>[4x]MKLSGVELRRVQMPLVAPFRTSFGTQSVRELLLLRAVTPAGEGWGECVTMAGPLYSSEYNDGAEHVLRHYLIPALLAAEDITAAKVTPLLAKFKGHRMAKGALEMAVLDAELRAHERSFAAELGSVR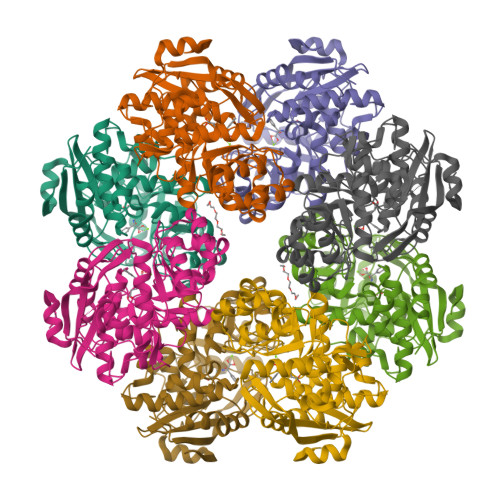DSVPCGVSVGIMDTIPQLLDVVGGYLDEGYVRIKLKIEPGWDVEPVRAVRERFGDDVLLQVDANTAYTLGDAPQLARLDPFGLLLIEQPLEEEDVLGHAELARRIQTPICLDESIVSARAAADAIKLGAVQIVNIKPGQVGGYLEARRVHDVCAAHGIPVWCGGMIETGLGRAANVALASLPNFTLPGDTSASDRFYKTDITEPFVLSGGHLPVPTGPGLGVAPIPELLDEVTTAKVWIGS>MSVLFISDLHLEAERPDITRAFLSFLDERARRAEALYILGDFFEAWIGDDGMDAFQRSIAQSLRQVADGGTRIYLMHGNRDFLIGKAFCREAGCTLLPDPSVIDLYGEPVLLMHGDSLCTRDEAYMRLRRWLRNPLTLWVLRHLPLATRHKLARKLRKESRAQTR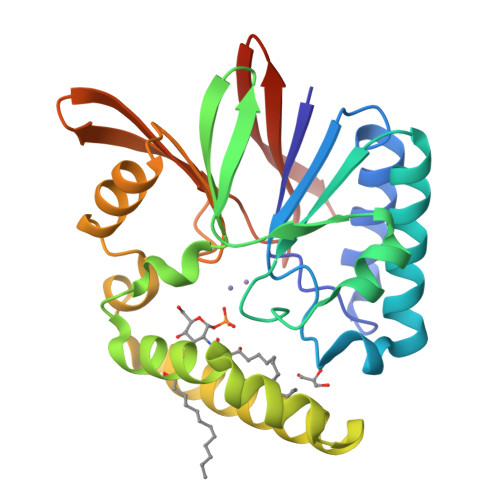MKAVDIIDVTPEEVPRVMRGHGVRTLIHGHTHRPAEHPLDIDGQPARRIVLGDWDRQGWALEIDANGHRQAPFPLLEHHHHHH[2x]>[2x]MSFIDPYQHIIVEHQYSHKFTVVVLRATKVTKGAFGDMLDTPDPYVELFISTTPDSRKRTRHFNNDINPVWNETFEFILDPNQENVLEITLMDANYVMDETLGTATFTVSSMKVGEKKEVPFIFNQVTEMVLEMSLEVCSCPDLRFSMALCDQEKTFRQQRKEHIRESMKKLLGPKNSEGLHSA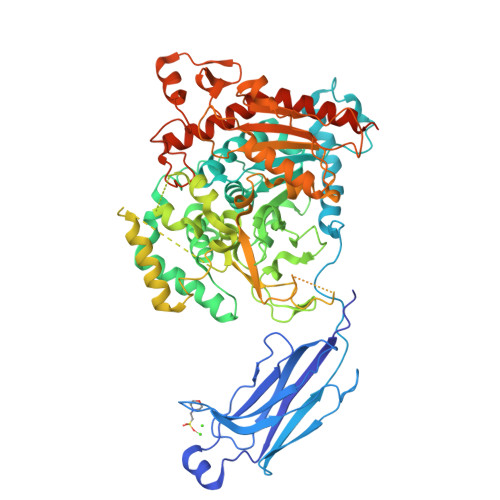RDVPVVAILGSGGGFRAMVGFSGVMKALYESGILDCATYVAGLSGSTWYMSTLYSHPDFPEKGPEEINEELMKNVSHNPLLLLTPQKVKRYVESLWKKKSSGQPVTFTDIFGMLIGETLIHNRMNTTLSSLKEKVNTAQCPLPLFTCLHVKPDVSELMFADWVEFSPYEIGMAKYGTFMAPDLFGSKFFMGTVVKKYEENPLHFLMGVWGSAFSILFNRVLGVSGSQSRGSTMEEELENITTKHIVSNDSSDSDDESHEPKGTENEDAGSDYQSDNQASWIHRMIMALVSDSALFNTREGRAGKVHNFMLGLNLNTSYPLSPLSDFATQDSFDDDELDAAVADPDEFERIYEPLDVKSKKIHVVDSGLTFNLPYPLILRPQRGVDLIISFDFSARPSDSSPPFKELLLAEKWAKMNKLPFPKIDPYVFDREGLKECYVFKPKNPDMEKDCPTIIHFVLANINFRKYKAPGVPRETEEEKEIADFDIFDDPESPFSTFNFQYPNQAFKRLHDLMHFNTLNNIDVIKEAMVESIEYRRQNPSRCSVSLSNVEARRFFNKEFLSKPKA> GSMADEATRRVVSEIPVLKTNAGPRDRELWVQRLKEEYQSLIRYVENNKNADNDWFRLESNKEGTRWFGKCWYIHDLL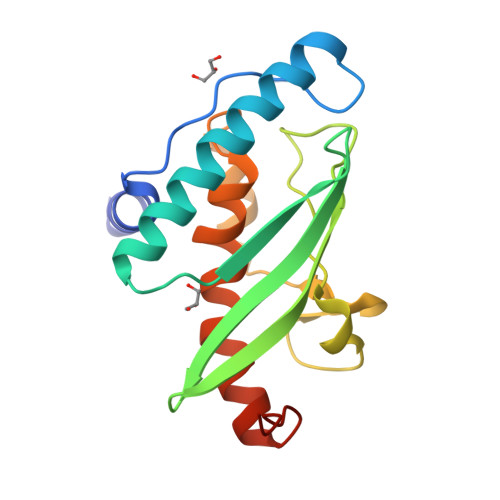KYEFDIEFDIPITYPTTAPEIAVPELDGKHPNMYRGGKICLTDHFKPLWARNVPKFGLAHLMALGLGPWLAVEIPDLIQKGVIHHKEKCNQ> GHMASGSLGELQESQSRLEAATKECQALEGRAR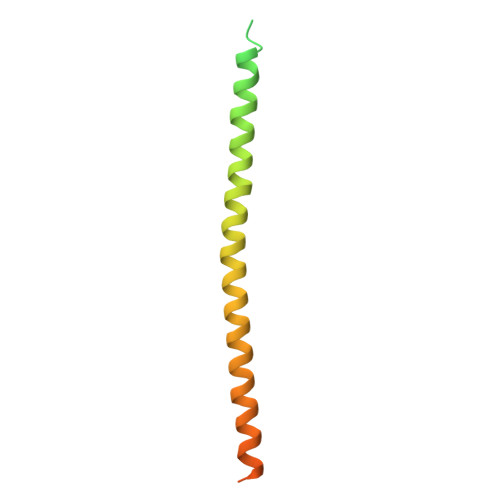AASEQARQLESEREALQQQHSVQVDQLRMQGQSVEAALRMERQAASEEKRKLAQLQVAYHQLFQEYDNHIKSSVVGSERKRGMQLEDLKQQLQQAEE The HAdV-D36 fiber knob domain (FK), which mediates the primary attachment of many HAdVs to host cells, has a significantly elongated DG loop that alters known binding interfaces for established adenovirus receptors such as the coxsackie- and adenovirus receptor (CAR) and CD46. Our data suggest that HAdV-D36 attaches to host cells using a versatile receptor pool comprising sialic acid-containing glycans and CAR. Sialic acids are recognized at the same binding site used by other HAdVs of species D such as HAdV-D37. Using glycan microarrays, we demonstrate that HAdV-D36 displays a binding preference for glycans containing a rare sialic acid variant, 4-O,5-N-diacetylneuraminic acid, over the more common 5-N-acetylneuraminic acid.

In contrast, HAdV-D37 showed preferential binding to 3’SL over 4-O-Ac-3’SL and bound to several other sialyl glycan probes in the array. In the case of the HAdV-D37 fiber knob, the two key polar interactions occur between residue K345 and the carboxyl group of Neu5Ac and between the backbone of P317 and the sugar’s amide nitrogen, respectively. In HAdV-D37, the N-acetyl group is accommodated in a canyon-shaped cavity formed mostly by two tyrosines (Y312 and Y308) from the neighboring monomer, as well as V322, which occupies the position analogous to F325. HAdV-D37, on the other hand, mediates only water-bridged contacts to the α-face. Interestingly, the O-acetyl function does not contribute any polar contact and instead induces the tilting movement under the steric influence of the bulky side chains of Y315 and P323. This interaction is supposedly not favorable for the binding; however, the steric constraints bring the O-acetyl groups of the three sugar moieties into a position in which they contact each other by means of a triangular hydrophobic interaction (mean distance between methyl C atoms: 4.3 Å) that displaces water molecules in the area. In the complex structure of HAdV-D37, the steric influence of the two residues Y312 and P320 is observable to the same extent, but the overall arrangement of the knob trimer does not allow the formation of this hydrophobic interaction (mean distance between methyl C atoms: 5.2 Å).

>[3x]MSKRLRVEDDFNPVYPYGYARNQNIPFLTPPFVSSDGFKNFPPGVLSLKLADPITITNGDVSLKVGGGLTLQDGSLTVNPKAPLQVNTDKKLELAYDNPFESSANKLSLKVGHGLKVLDEKSAAGLKDLIGKLVVLTGKGIGTENLENTDGSSRGIGINVRAREGLTFDNDGYLVAWNPKNDTRTLWTTPDTSPNCTIAQDKDSKLTLVLTKCGSQILANVSLIVVAGKYHIINNKTNPKIKSFTIKLLFNKNGVLLDNSNLGKAYWNFRSGNSNVSTAYEKAIGFMPNLVAYPKPSNSKKYARDIVYGTIYLGGKPDQPAVIKTTFNQETGCEYSITFNFSWSKTYENVEFETTSFTFSYIAQE> GPLGSN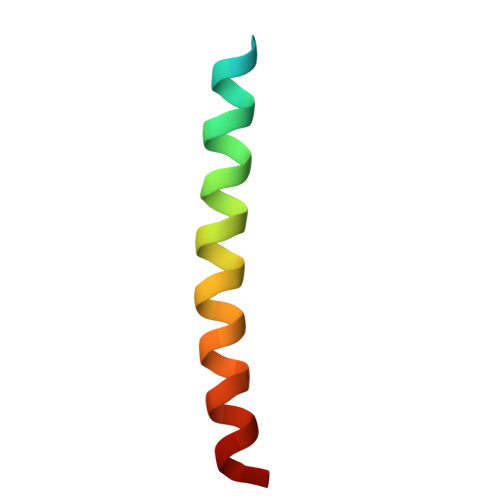RRLQQTQAQVDEVVDIMRVNVDKVLERDQKL> TDGNAGLLAEPQIAMFCGRLNMHMNVQNGKWDSDPSGTKTCIDTKEGILQYCQEVYPELQITNVVEANQPVTIQNWCKRGRKQCKTHPHFVI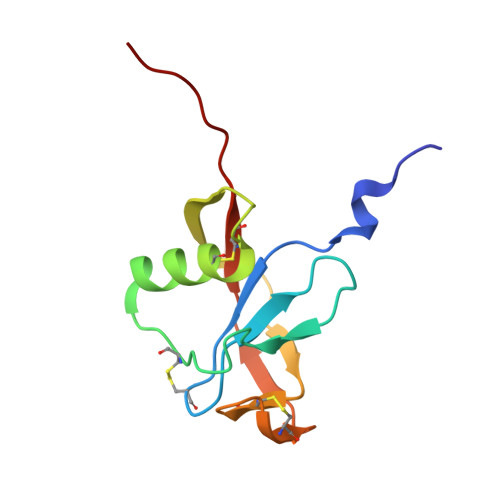PYRCLVGEFVSDA> CAAELAALEAELAALEGPWKGYPIPYGKL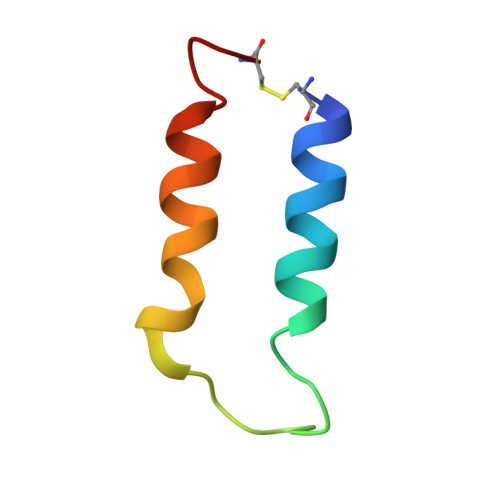QFLIKKLKQLKVAC> MELQEVLHMNGGEGDTSYAKNSSYNLFLIRVKPVLEQCIQELLRANLPNINKCFKVGDLGCASGPNTFSTVRDIVQSIDKVGQEKKNELERPT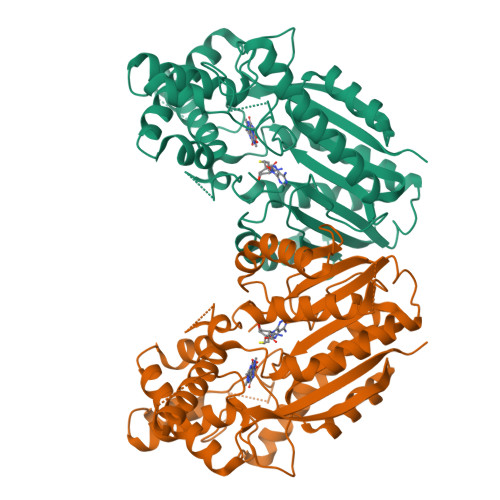IQIFLNDLFQNDFNSVFKLLPSFYRNLEKENGRKIGSCLIGAMPGSFYSRLFPEESMHFLHSCYCLHWLSQVPSGLVTELGISVNKGCIYSSKASRPPIQKAYLDQFTKDFTTFLRIHSEELISRGRMLLTFICKEDEFDHPNSMDLLEMSINDLVIEGHLEEEKLDSFNVPIYAPSTEEVKRIVEEEGSFEILYLETFNAPYDAGFSIDDDYQGRSHSPVSCDEHARAAHVASVVRSIYEPILASHFGEAILPDLSHRIAKNAAKVLRSGKGFYDSVIISLAKKPEKADM>MASGGAFCLIANDGKADKIILAQDLLNSRISNIKNVNKSYGKPDPEPTLSQIEETHLVHFNAHFKPYVPVGFEYNKVRPHTGTPTLGNKLTFGIPQYGDFFHDMVGHHILGACHSSWQDAPIQGTSQMGAHGQLQTFPRNGYDWDNQTPLEGAVYTLVDPFGRPIVPGTKNAYRNLVYYCEYPGLRLYENVRFEVNGNSLDEYSSDVTTLVRKFCIPGDKMTGYKHLVGQEVSVEGTSGPLLCNIHDLHKPHQSKPILTDENDTQRTCSHTNPKFLSQHFPHFPENIQTAGKQDITPITDATYLDIRRNVHYSCNGPQTPKYYQPPLALWIKLRFWFNDNVNLAIPSVSIPFGERFITIKLASQKDLVNEFPGLFVRQSTVIAGRPSRRNIRFKPWFIPGVINEISLTNNELYINNLFVTPEIHNLYVKRVRFSLIRVHKTQVTHTNNNHHDEKLMSALKWPIEYMFIGLKPTWNISDQNPHQHRDWHKFGHVVNAIMQPTHHAEISFQDRDTALPDACSSISDISPVTYPITLPIIKNISVTAHGINLIDKFPSQFCSSYIPFHY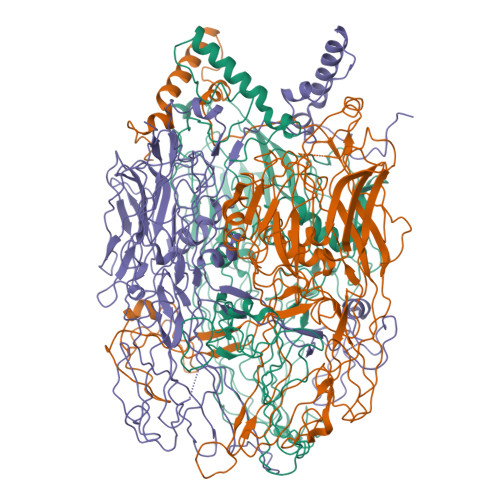GGNAIKTPDDPGAMMITFALYPREEYQPSGHINVSRAREFYISWDSDYVGSITTADLVVSSSAINFLLLQNGSAVLRYST[3x]>QNSLALHKVIMVGSGGVGKSALTLQFMYDEFVEDYEPTKADSYRKKVVLDGEEVQIDILDTAGLEDYAAIRDNYFRSGEGFLCVFSITEMESFAATADFREQILRVKEDENVPFLLVGNKSDLEDKRQVSVEEAKNRAEQWNVNYVETSAKTRANVDKVFFDLMREIR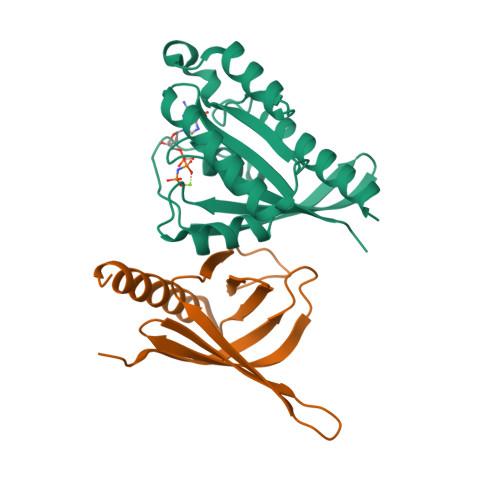ARKMEDS[2x];>LETPGQYLVYNGDLVEYEADHMAQLQRVHGFLMNDCLLVATWLPQRRGMYRYNALYPLDRLAVVNVKDNPPMKDMFKLLMFPESRIFQAENAKIKREWLEVLEETKRALSDKR[2x]> GFPTELKPGTNQFLTTDDGVSAPILPNFHPTPCIHIPGEVRNLLELCQ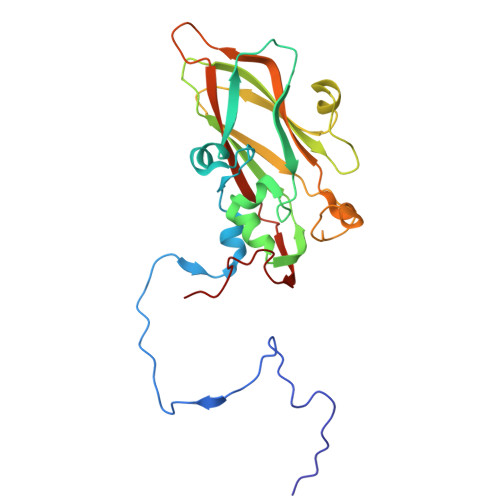VETILEVNNVPTNATSLMERLRFPVSAQAGKGELCAVFRADPGRSGPWQSTLLGQLCGYYTQWSGSLEVTFMFTGSFMATGKMLIAYTPPGGPLPKDRATAMLGTHVIWDFGLQSSVTLVIPWISNTHYRAHARDGVFDYYTTGLVSIWYQTNYVVPIGAPNTAYIIALAAAQKNFTMKLCKDASDILQTGTIQ>[2x]MGSMATLKAQHLAKSYKGRQVVRDVSMSIDSGQIVGLLGPNGAGKTTCFYMIVGLVQADQGVVRIDEQNVTHLPMHGRARAGIGYLPQEASIFRKLSVSDNIMAILETRSDLDRNGRKEALEGLLQEFHIHHIRDNLGMSLSGGERRRVEIARALASAPKFILLDEPFAGVDPISVGDIKQIIHHLKAKGIGILITDHNVRETLDICETAYIVNDGQLIAEGDAESILANDLVKEVYLGHEFRLKLHHHHHH;> MGSMPKTLRQKLLLALIALLLIVAGYYWNVGLELFNEQPTRPGQDNTIDYYAENAHSLQYQEDGSLDYEMTAVKLEHQKATDITFVTTPDLLLFRGNVQPWHIQSARAEVGPKGKEVELIDDVRVARTDAKGQPSILTTTRLTVFPDKNYAQTEQAVKIDAANGVTTAVGMKAYLKDSRMHLLSNVRGQHEVR;> MGSMIVFRYLSREVLVTMSAVSAVLLVIIMSGRFIKYLAQAAQGLLDPGSLFLIMAFRIPGFLQLILPLGLFLGILLAYGRLYLESEMTVLSATGMSQKRLLGYTMAPALLVAILVAWLSLFLAPQGINQFALLLNKQDTLTEFDTLVPGRFQAMRDGTRVTYTEELSKDRGELAGIFISQKDLNSSNQERGISILVAEKGTQNIQADGSRYLILHNGYRYDGNPGQANYRAIQYDTYGVMLPKPEASSEVSERDAVPTADLFGSDNPRYQAELQWRLSTPLLVFVVTLLAVPLSRVNPRQGRFLKLLPAILLYMGYLALLIAVRGQLDKGKIPMAIGLWWVHGLFLAIGLLLFYWEPLRLKLASSRAGREVAHG;> MGSMVKLDRYIGVTVFVAILAVLGVILGLALLFAFIDELNDISASYGIGDALRFIFLTAPRRAYDMLPMAALIGCLVGLGTLASNSELTIMRAAGVSLSRIVWAVMKPMLVLMLAGILVGEYVAPWTENIAQSGRALAQGGGDSQSSKRGLWHRQGREYIHINAVQPNGVLYGVTRYRFDEQRGLESASFAKRARFETDHWQLEEVTTTLLHPREKRSEVVKLPTERWDAQLSPQLLNTVVMEPEALSISGLWQYIHYLADQGLNNNRYWLAFWTKVLQPLVTAALVLMAISFIFGPLRSVTLGQRIFTGVLVGFVFRIAQDLLGPSSLVFDFPPLLAVVIPASICALAGVWLLRRAG

The IM sub-complex comprises the ATP-binding cassette (ABC) transporter LptB2FGC, which extracts LPS from the IM and delivers it to the periplasmic components of the Lpt system. LptB2FGC is a type VI ABC transporter consisting of 5 subunits. The LptB cytoplasmic subunits form the nucleotide-binding domains (NBDs) that capture and hydrolyse ATP. LptF and LptG possess transmembrane helices that create a cavity and a translocation path for LPS, as well as a periplasmic β-jellyroll domain.

We also obtained two cryo-EM 3D reconstitutions of LptB2FGC at resolutions of 3.26 Å and 3.61 Å, respectively. These two structures were assigned as LptB2FGC-I and LptB2FGC-II. Structure alignment of these two structures gives rise to a root mean square deviation (RMSD) of 1.2 Å over 1324 Cα atoms and indicates the main difference between these two cryo-EM structures is in the β-jellyroll structures. These regions appear to perform a rigid body rotation motion toward the outer leaflet of IM, similarly to what we observed for LptB2FG. The TMD and NBD domains of LptB2FGC are similar to those of the LptB2FG structures and represent the resting state. In our LptB2FGC structures, the periplasmic β-jellyroll of LptC was clearly resolved and found to form a trimeric interface: LptC and LptF form the primary LPS transfer path, while a loop from LptG (residues 209–215) binds onto the N-terminal β-jellyroll of LptC (residues 60–69). Intriguingly, in contrast to previously documented LptB2FGC structures, the transmembrane helix of LptC remained unobservable in these maps, indicating its flexibility and a lack of engagement with LptF and LptG at Interface 1. This, in turn, results in an unobstructed entry point for LPS into the TMD cavity. Similar to LptB2FG, we identified four lipids in the transmembrane region of the form I conformation, which likely originate from nanodisc reconstitution. However, for LptB2FGC-II, the lower resolution and particle counts in this conformation prevented confident lipid identification.> MSNEEFTQLMLEALDGFFLAIMTDGSIIYVSESVTSLLEHLPSDLVDQSIFNFIPEGEHSEVYKILSTHLLESDSLTPEYLKSKNQLEFCCHMLRGTIDPKEPSTYEYVKFIGNFKSLNS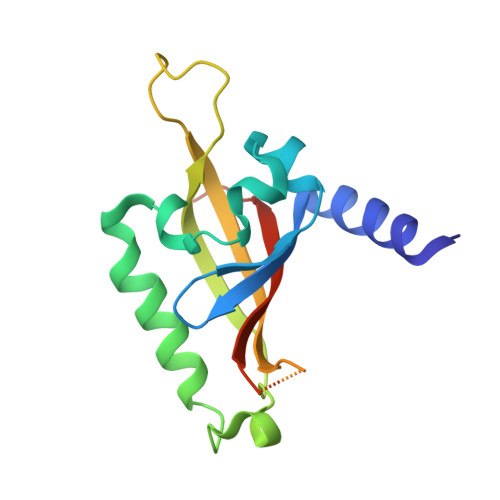VSSSAHNGFEGTIQRTHRPSYEDRVCFVATVRLATPQFIKE> MRLRRLYCRTGGFHLQILPDGRVDGTREDNSPYSLLEIRAVEVGVVAIKGVKSGRYLAMNKKGRLYGSKHFTDECKFKERLLENGYNTYSSAKYRRGWYVALNKNGRPKK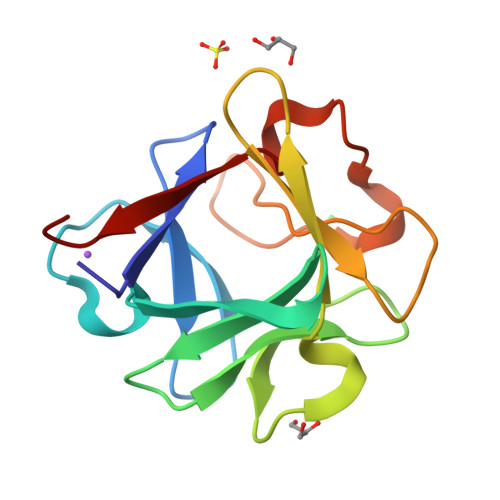GNRTRRTQKATHFLPLPVSG>[16x]GGDGNITTENIPVSEYDCLELEGGGMVVNYTQSDAPEGLEIKTDRNIFEKYEFNVENHKLKIRPKKEFRKHTNFRPTEFMVTANSRNLKKL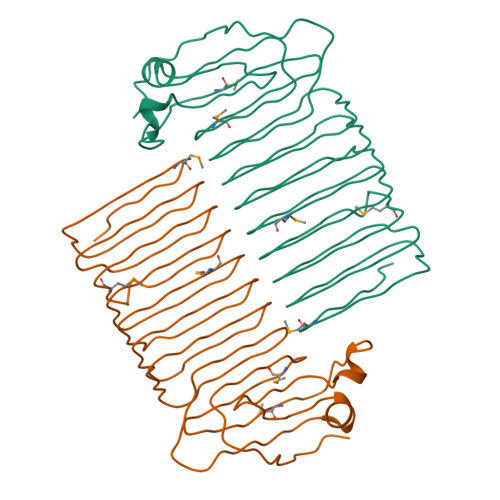AAAGSTHVNINSPLQAEEFEAGLAGSGIIQFHDTASFTNLKIEIAGSGDFVGHKVYCEELNGDMAGSNTIVLGGTVGIAEFSIAGSGTVRAFDCTMDELECKIAGSGDIEAFVVNKIKAEIAGSGSVKYKGDPQDIQKKVMGSGKIEKVE> SADAQSFLNRVCGVSAARLTPCGTGTSTDVVYRAFDIYNDKVAGFAKFLKTNCCRFQEKDEDDNLIDSYFVVKRHTFSNYQHEETIYNLLKDCPAVAKHDFFKFRIDGDMVPHISRQRLTKYTMADLVYALRHFDEGNCDTLKEILVTYNCCDDDYFNKKDWYDFVENPDILRVYANLGERVRQALLKTVQFCDAMRNAGIVGVLTLDNQDLNGNWYDFGDFIQTTPGSGVPVVDSYYSLLMPILTLTRALTAESHVDTDLTKPYIKWDLLKYDFTEERLKLFDRYFKYWDQTYHPNCVNCLDDRCILHCANFNVLFSTVFPPTSFGPLVRKIFVDGVPFVVSTGYHFRELGVVHNQDVNLHSSRLSFKELLVYAADPAMHAASGNLLLDKRTTCFSVAALTNNVAFQTVKPGNFNKDFYDFAVSKGFFKEGSSVELKHFFFAQDGNAAISDYDYYRYNLPTMCDIRQLLFVVEVVDKYFDCYDGGCINANQVIVNNLDKSAGFPFNKWGKARLYYDSMSYEDQDALFAYTKRNVIPTITQMNLKYAISAKNRARTVAGVSICSTMTNRQFHQKLLKSIAATRGATVVIGTSKFYGGWHNMLKTVYSDVENPHLMGWDYPKCDRAMPNMLRIMASLVLARKHTTCCSLSHRFYRLANECAQVLSEMVMCGGSLYVKPGGTSSGDATTAYANSVFNICQAVTANVNALLSTDGNKIADKYVRNLQHRLYECLYRNRDVDTDFVNEFYAYLRKHFSMMILSDDAVVCFNSTYASQGLVASIKNFKSVLYYQNNVFMSEAKCWTETDLTKGPHEFCSQHTMLVKQGDDYVYLPYPDPSRILGAGCFVDDIVKTDGTLMIERFVSLAIDAYPLTKHPNQEYADVFHLYLQYIRKLHDELTGHMLDMYSVMLTNDNTSRYWEPEFYEAMYTPHTVLQHHHHHHHHHH;>AIASEFSSLPSYAAFATAQEAYEQAVANGDSEVVLKKLKKSLNVAKSEFDRDAAMQRKLEKMADQA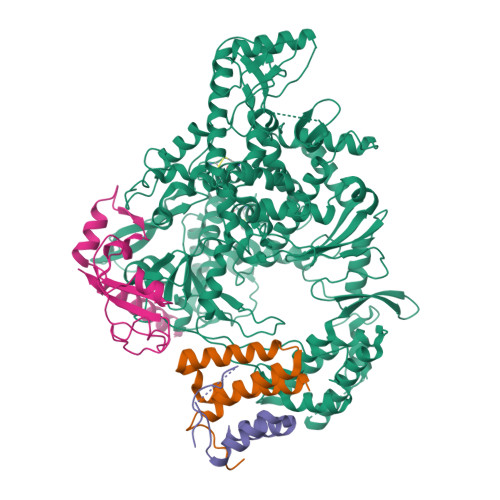MTQMYKQARSEDKRAKVTSAMQTMLFTMLRKLDNDALNNIINNARDGCVPLNIIPLTTAAKLMVVIPDYNTYKNTCDGTTFTYASALWEIQQVVDADSKIVQLSEISMDNSPNLAWPLIVTALRANSAVKLQ[2x];> SKMSDVKCTSVVLLSVLQQLRVESSSKLWAQCVQLHNDILLAKDTTEAFEKMVSLLSVLLSMQGAVDINKLCEEMLDNRATLQ>FQPGDRIEVLNGEQRGSKGIVTRTTKDIATIKLNGFTTPLEFPISTLRKIFEPGDHVTVINGEHQGDAGLVLMVEQ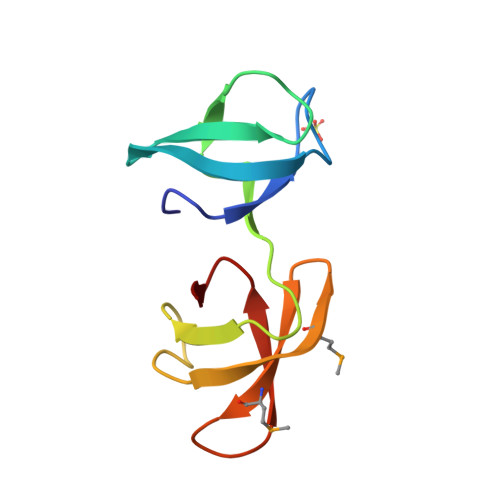GQVTFMSTQTSREVTITANNLSK[2x]> TSSANEDMPVERILEAELAVEPKTETYVEANMGLNPSSPNDPVTNICQAADKQLFTLVEWAKRIPHFSELPLDDQVILLRAGWNELLIASFSHRSIAVKDGILLATGLHVHRNSAHSAGVGAIFDRVLT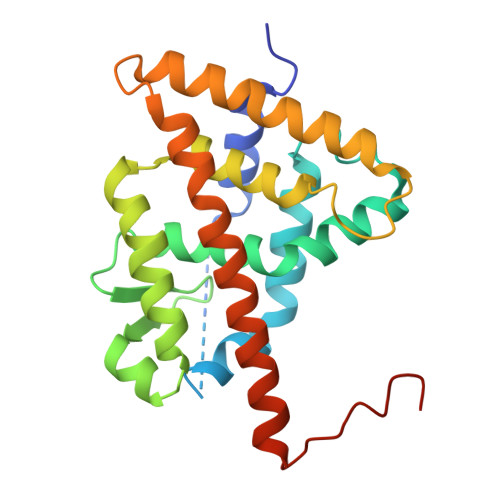ELVSKMRDMQMDKTELGCLRAIVLFNPDSKGLSNPAEVEALREKVYASLEAYCKHKYPEQPGRFAKLLLRLPALRSIGLKCLEHLFFFKLIGDTPIDTFLMEMLEAPHQMT> GSMGKDEALEKDLNDVSKEINLMLSTYAKLLSERAAVDASYIDEIDELFKEANAIENFLIQKREFLRQ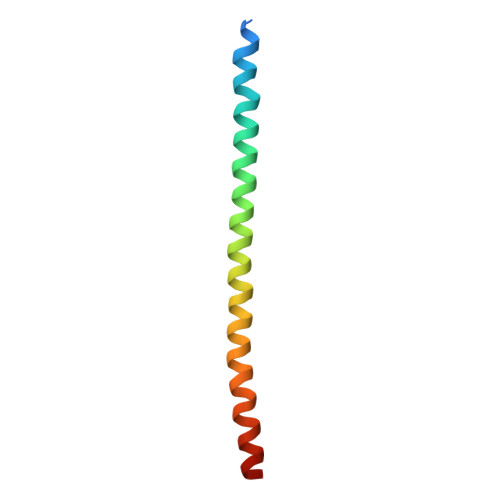R(2S,3R,4Z)-3-hydroxy-2-[(9E)-octadec-9-enoylamino]octadec-4-en-1-yl dihydrogen phosphate 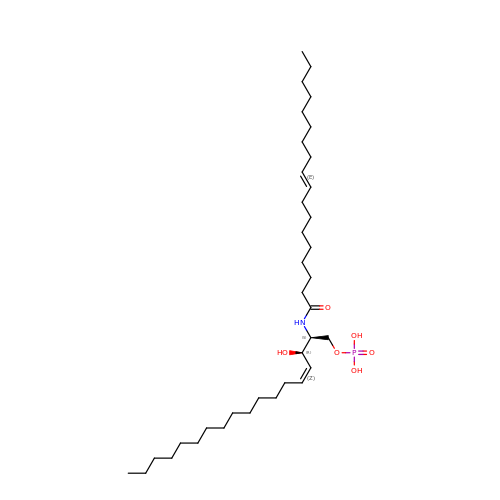| C36 H70 N O6 P | HOOJDMQIUTXSPU-GINUSHNTSA-N>[2x]MAEQVLPQALYLSNMRKAVKIRERTPEDIFKPTNGIIHHFKTMHRYTLEMFRTCQFCPQFREIIHKALIDRNIQATLESQKKLNWCREVRKLVALKTNGDGNCLMHATSQYMWSVQDTDLVLRKALFSTLKETDTRNFKFRWQLESLKSQEFVETGLCYDTRNWNDEWDNLIKMASTDTPMARSGLQYNSLEEIHIFVLCN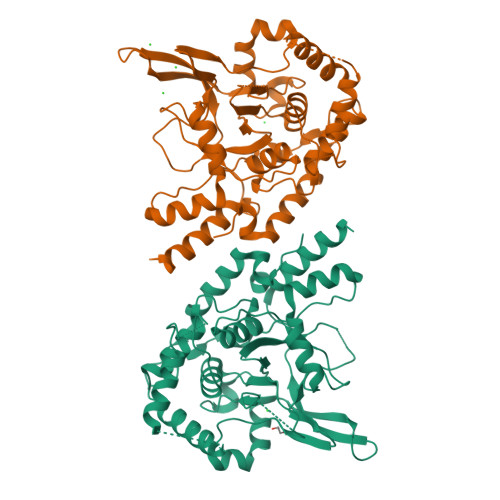ILRRPIIVISDKMLRSLESGSNFAPLKVGGIYLPLHWPAQECYRYPIVLGYDSHHFVPLVTLKDSGPEIRAVPLVNRDRGRFEDLKVHFLTDPENEMKEKLLKEYLMVIEIPVQGWDHGTTHLINAAKLDEANLPKEINLVDDYFELVQHEYKKWQENSEQGRRE>[10x]MEGLNLVATALAVGLGAIGPGVGIGIIVSGAVQAIGRNPEIENRVVTYMFIGIAFTEALAIFGLVIAFLIGFGVLQ;>[2x]MSTRTRNILIIVGALIISIASRFFLYTGPPHVEVAAEVIFDGIPGFPITNSFVVAIIIDIFVIALAVAATRNLQMVPRGLQNVMEFILESLYNLFRNINAKYVATAFPLVATIFLFVLFGNWFGLLPGVGSIGVCHEKKEEHAVVDERLALAAPAAPLSSVAAAEGEEIHDTCAAQGKKLVPLFRAPAADLNFTFAIAVISFVFIEYWGFRALGPGYLKKFFNTNGIMSFVGIIEFISELVKPFALAFRLFGNIFAGEVLLVVMAFLVPLLLPLPFYGFEVFVGFIQALIFALLTYAFLNIAVTGHDEEHAH;>MEALGINP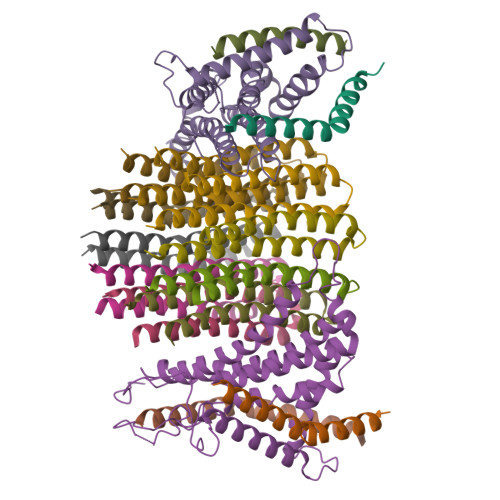TLFIAQLINFLLLIFILRALLYRPVMNLLNERTRRIEESVRDAEKVREQLANARRDYEAEIARARQEAAKIVAQAQERAKQQEAEIIAQARREAERLKEEARAQAEQERIRMLSEAKSQIADLVTLTASRVLGAELQARGHDALIAESLAALDRRN[4x]In Arabidopsis, the SRA domain of the SU(VAR)3-9 HOMOLOG (SUVH) histone methyltransferase recognizes 5 mC (mC) in different sequence contexts and methylation statuses. The recognition of methylated DNA is required for the maintenance of the repressive marks 5 mC and histone H3 lysine dimethylation (H3K9me2), and for silencing the transposable elements and gene transcription in plants. Our studies are the first to establish that SUVH5 SRA specifically binds 5 mC and 5 hmC bases, but exhibits weaker affinities towards 5 fC and 5 caC modified bases. SUVH5 is unusual among the SRA domain proteins, as its SRA domain efficiently binds methylated and hydroxymethylated CG DNA, as well both the hemi- and fully modification statuses.

To understand the molecular mechanisms of SUVH5 SRA-mediated recognition of fully-5 hmCG DNA, we determined the crystal structure of SUVH5 SRA in a complex with a self-complementary 10-base pair duplex containing centrally located 5 hmC-G pairs with a 3′ “T” overhang. The biological assembly of the complex, two SRA molecules bound to duplex DNA, is generated by the crystallographic two-fold axis perpendicular to the DNA helical-axis. The symmetrical 5 hmC bases from the adjacent base pairs are flipped out and positioned in the binding pocket of individual SRA molecules. Gln392, located on the thumb loop (connects α1-helix and β2-strand), inserts into the minor groove and substitutes for the flipped out 5 hmC in the duplex DNA. In addition, Gln392 forms intermolecular hydrogen bonds with the Watson-Crick edge of the orphan guanine and stacking interactions with the flanking bases, thereby compensating for the extrusion of the 5 hmC bases from the DNA double helix. The flipped out 5 hmCs are tightly positioned in the pocket via parallel-displaced π-stacking interactions with Tyr416 and Tyr428, and by intermolecular hydrogen bonds between its Watson-Crick edge and the side chain of Asp418. The hydroxyl group of 5 hmC participates in intermolecular interactions with the side chain of Tyr428 and the main chain nitrogen of Gly394 from the thumb loop. Our structural analysis revealed that the flipped-out 5 hmC adopts a similar conformation in the binding pocket and has a similar distribution of intermolecular interactions as that of the flipped-out 5 mC in the crystal structure of the SUVH5 SRA-fully-5 mCG complex. 5 hmC binding induces a conformational change in the pocket, and the wall region (Gly414-Asp418) is reorganized to accommodate bases larger than 5 mC. The penalty for accommodating a larger base, 5 hmC, in the binding pocket may be compensated by the hydroxyl group specific interactions, thereby accounting for the insignificant difference in the binding affinity between fully-5 mCG and fully-5 hmCG for SUVH5 SRA.

> QIIGTVPGVEVGDEFQYRMELNLLGIHRPSQSGIDYMKDDGGELVATSIVSSGGYNDVLDNSDVLIYTGQGGNVGKKKNNEPPKDQQLVTGNLALKNSINKKNPVRVIRGIKNTTLQSSVVAKNYVYDGLYLVEEYWEETGSHGKLVFKFKLRRIPGQPELPWKEVA>MLSYRHSFHAGNHADVLKHTVQSLIIESLKEKDKPFLYLDTHAGAGRYQLGSEHAERTGEYLEGIARIWQQDDLPAELEAYINVVKHFNRSGQLRYYPGSPLIARLLLREQDSLQLTELHPSDYPLLRSEFQKDSRARVEKADGFQQLKAKLPPVSRRGLILIDPPYEMKTDYQAVVSGIAEGYKRFATGIYALWYPVVLRQQIKRMIHDLEATGIRKILQ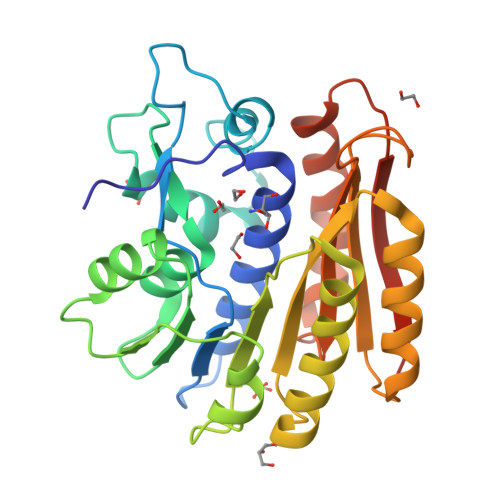IELAVLPDSDRRGMTASGMIVINPPWKLEQQMNNVLPWLHSKLVPAGTGHATVSWIVPESKGHHHHHH[2x]> GMAHPPQIRIPATYLRGGTSKGVFFRLEDLPESCRVPGEARDRLFMRVIGSPDPYAAHIDGMGGATSSTSKCVILSKSSQPGHDVDYLYGQVSIDKPFVDWSGNCGNLSTGAGAFALHAGLVDPARIPEDGICEVRIWQANIGKTIIAHVPVSGGQVQETGDFELDGVTFPAAEIVLEFLDPSDDGEDGGAIFPTGNLVDDLEVPGV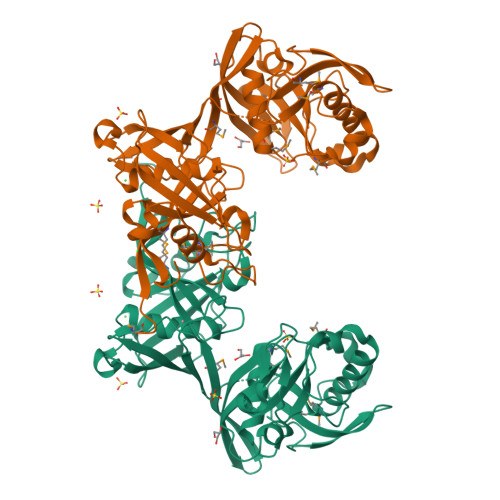GTFKATMINAGIPTVFVNAEEIGYRGTELREEINGDPQQLARFERIRVAGALRMGLIKTPEEAATRQHTPKIAFVAPPRDYRTASGKLVAAGDIDLLVRALSMGKLHHAMMGTAAVAIGTAAAIPGTLVNLAAGGGERSAVRFGHPSGTLRVGAEASQANGEWTVTKAIMSRSARILMEGWVRVPGDAF> MAPSRLCVYCADVCPDRLRCAAWLLATGIFLLLAGCSEAKAPTALERVQKEGVLRVITRNSPATYFQDRNGETGFEYELAKRFAERLGVELKIETADNLDDLYAQLSREGG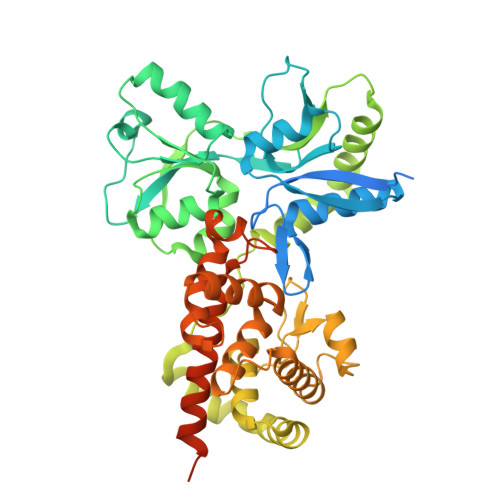PALAAAGLTPGREDDASVRYSHTYLDVTPQIIYRNGQQRPTRPEDLVGKRIMVLKGSSHAEQLAELKKQYPELKYEESDAVEVVDLLRMVDVGDIDLTLVDSNELAMNQVYFPNVRVAFDFGEARGLAWALPGGDDDSLMNEVNAFLDQAKKEGLLQRLKDRYYGHVDVLGYVGAYTFTQHLQQRLPRYESHFKQSGKQKDTDWRLLAAIGYQESLWQPGATSKTGVRGLMMLTNRTAQAMGVSNRLDPKQSIQGGSKYFVQIRSELPESIKEPDRSWFALAAYNIGGAHLEDARKMAEKEGLNPNKWLDVKKMLPRLAQKQWYAKTRYGYARGGETVHFVQNVRRYYDILTWVTQSQMEGSQIAESGLHLPGVNKTRPEEDSGDEKL>MSQPITRENFDEWMIPVYAPAPFIPVRGEGSRLWDQQGKEYIDFAGGIAVNALGHAHPELREALNEQASKFWHTGNGYTNEPVLRLAKKLIDATFADRVFFCNSGAEANEAALKLARKFAHDRYGSHKSGIVAFKNAFHGRTLFTVSAGGQPAYSQDFAPLPADIRHAAYNDINSASALIDDSTCAVIVEPIQGEGGVVPASNAFLQGLRELCNRHNALLIFDEVQTGVGRTGELYAYMHYGVTPDLLTTAKALGGGFPVGALLATEECARVMTVGTHGTTYGGNPLASAVAGKVLELINTPEMLNGVKQRHDWFVERLNTINHRYGLFSEVRGLGLLIGCVLNADYAGQAKQISQEAAKAGVMVLIAGGNVVRFAPALNVSEEEVTTGLDRFAAACEHFVSRGSS[2x]

Escherichia coli possesses two acyl ornithine aminotransferases, one catabolic (AstC) and the other anabolic (ArgD), that participate in L-arginine metabolism. The arginine-succinyl transferase pathway of E. coli provides nitrogen for growth via a series of succinylated intermediates. In conclusion, the E. coli AstC protein, involved in arginine catabolism, is a PLP containing transaminase that is structurally similar to the related protein ArgD, which is the transaminase enzyme used in arginine synthesis. From the biochemical data, it appears that AstC and ArgD are biochemically similar, consistent with the ability of astC to complement an argD deletion. Both have comparable steady state kinetic values, with a strong preference for the acylated ornithine derivatives AO (AstC and ArgD) and SO (for AstC, at least) over ORN itself.

The native, non-tagged AstC that was purified from E. coli was the apo-protein, with no bound PLP, as suggested by the lack of color of the purified protein, and confirmed by a UV-Vis absorbance spectrum, which showed no absorbance in the region of 320 to 500 nm (data not shown) which is characteristic of PLP containing proteins. We were able to obtain crystals of the apo-protein, although they diffracted to only medium resolution (2.75 Å). Consistent with our spectrophotometric data, there was no electron density for the PLP co-factor in the crystal structures of protein obtained directly from purification. The A and B protomers in the asymmetric unit differ substantially, with the A chain having electron density for almost the entire length of the molecule (Gln3 to Ser402) and the B chain starting at residue Ala21 and ending at Ser402. The B chain also has no electron density corresponding to two loops in the A chain from His142 to Ala163 and Val274 to Gly283, respectively. The two protomers do not form a dimer, rather dimers are formed through crystallographic symmetry for both, the A with another A protomer and the B with another B protomer. The loops missing from the B protomer form part of the dimer interface; analysis of the PISA output shows that the A–A interface buries about 4763 Å2 whereas the B–B interface buries only 1906 Å2. The St-ArgD structures are most similar to the B protomer of the apo-enzyme structure of AstC reported here, in that the N-terminal ∼23 amino acids of the structures are missing as are six residues in a loop from 277–282. The reconstituted enzyme was more heat stable than the apo-protein; holo-AstC and apo-AstC had apparent Tm values of 46°C and 43.5°C, respectively.>MAVPETRPNHTIYINNLNEKIKKDELKKSLYAIFSQFGQILDILVSRSLKMRGQAFVIFKEVSSATNAL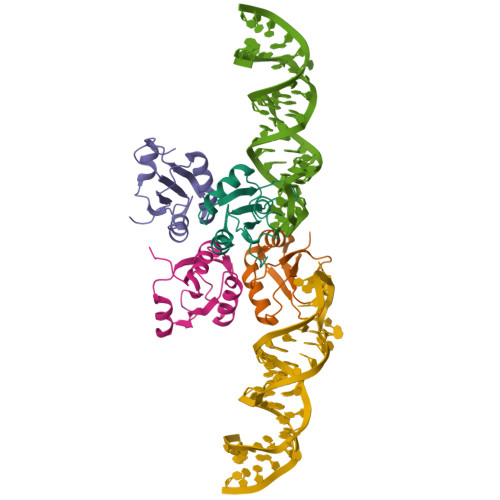RSMQGFPFYDKPMRIQYAKTDSDIIAKMKGTFV[4x]[(S)-(4-fluorophenyl)-[[(2S)-2-methyl-3-sulfanyl-propanoyl]amino]methyl]boronic 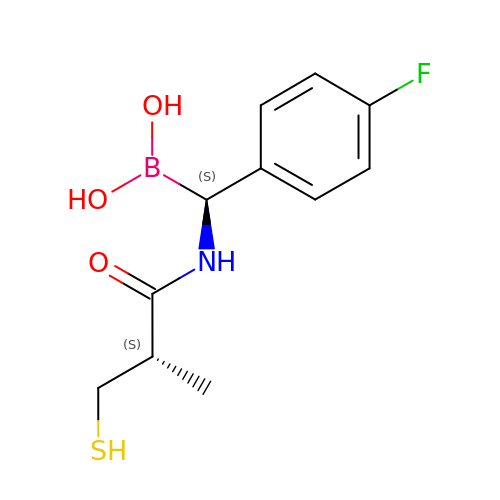acid | C11 H15 B F N O3 S | CDDJMEDWZMPIRW-GMSGAONNSA-N>[2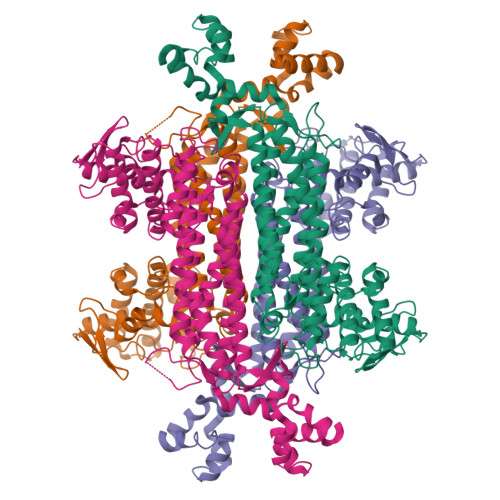x]MEYRIERDTMGEVRVPADKYWGAQTQRSLENFRIGTDRFRMPLEIIRAYGMLKKAAARANLELGELPEEIAKAIIQAAEEVVQGKWDDHFPLVVFQTGSGTQTNMNVNEVIANRASEILGKPLGSKYAHPNDHVNRGQSSNDTFPTAMYVAVALALHQRLYPAVEGLIRTFTAKAQAFDQIVKVGRTHLMDAVPITLGQEIGSWAAQLKTTLAAVKEMEKGLYNLAIGGTAVGTGLNAHPRFGELVAKYLAEETGLPFRVAENRFAALAAHDELVNVMGAIRTLAGALMKIGNDVRWLASGPYAGIGEITIPANEPGSSIMPGKVNPTQVEALTMVVVRVYGNDHTVAFAGSQGNFQLNVYKPVMAYSTLESINLLADAVASFDAHLAQGIEPNLERIEEYLQKNPMLATALNKAIGYDKAAEIVKKALKEKKTLKQAALELGYLTEEEFDRIVVPMRLAKPHEGA>[2x]SNAMISHIGTIDV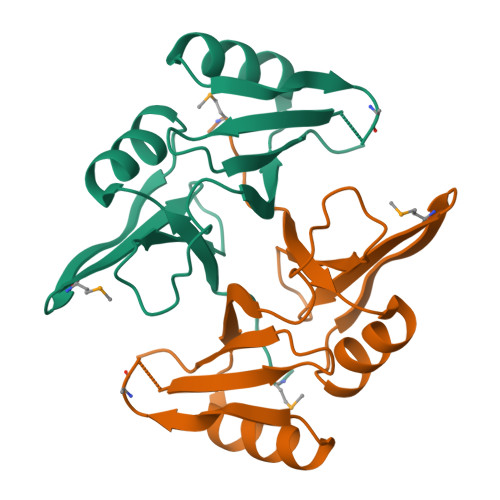FVNDQDKAIDFYVNTLGFELREDQAFGPMRWVEVAPAGSQTRIVLCTKHFPVYEEGKIGRFTDIQLVTEDIKATHEELVRRGVNFTRAPEQMPFGGANASFQDPDGNEFLLLQPSR> AEAGITGTWYNQLGSTF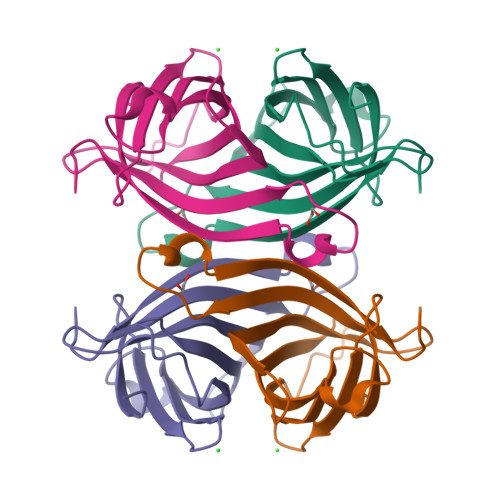IVTAGADGALTGTYESAVGNAESRFVLTGRYDSAPATDGSGTALGWTVAWKNNYRNAHSATTWSGQYVGGAEARINTQWLLTSGTTEANAWKSTLVGHDTFTKVKPSAAS>[2x]MVRDMKHTVEVMIPEAEIKARIAELGR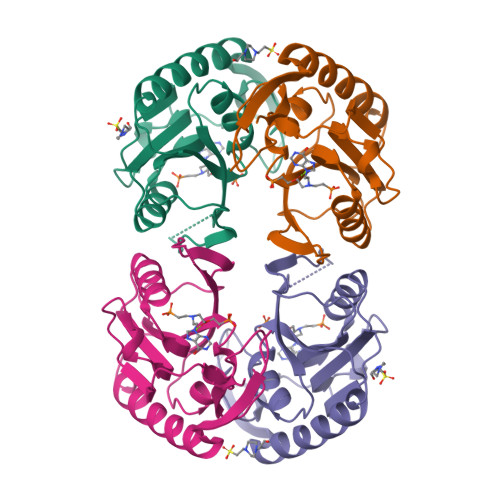QITERYKDSGSDMVLVGLLRGSFMFMADLCREVQVSHEVDFMTASSYGSGMSTTRDVKILKDLDEDIRGKDVLIVEDIIDSGNTLSKVREILSLREPKSLAICTLLDKPSRREVNVPVEFIGFSIPDEFVVGYGIDYAQRYRHLPYIGKVILLDE> YSIEADKKFKYSVKLSDYPTLQDAASAAVDGLLIDRDYNFYGGETVDFGGKVLTIECKAKFIGDGNLIFTKLGKGSRIAGVFMESTTTPWVIKPWTDDNQWLTDAAAVVATLKQSKTDGYQPTVSDYVKFPGIETLLPPNAKGQNITSTLEIRECIGVEVHRASGLMAGFLFRGCHFCKMVDANNPSGGKDGIITFENLSGDWGKGNYVIGGRTSYGSGSSAQFLRNNGGFERDGGVIGFTSYRAGESGVKTWQGTVGSTTSRNYNLQFRDSVVIYPVWDGFDLGADTDMNPELDRPGDYPITQYPLHQLPLNHLIDNLLVRGALGVGFGMDGKGMYVSNITVEDCAGSGAYLLTHESVFTNIAIIDTNTKDFQANQIYISGACRVNGLRLIGIRSTDGQGLTIDAPNSTVSGITGMVDPSRINVANLAEEGLGNIRANSFGYDSAAIKLRIHKLSKTLDSGALYSHINGGAGSGSAYTQLTAISGSTPDAVSLKVNHKDCRGAEIPFVPDIASDDFIKDSSC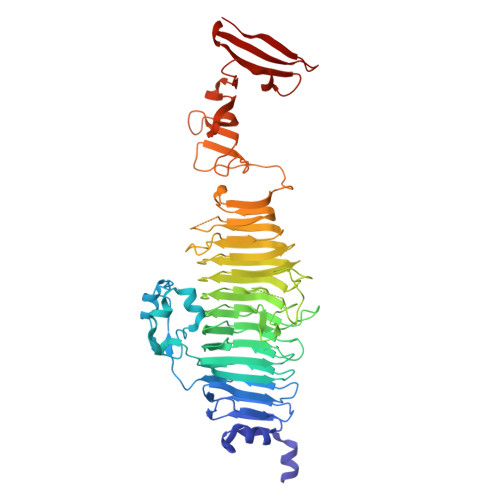FLPYWENNSTSLKALVKKPNGELVRLTLATL(2-NAPHTHALEN-2-YL-1-NAPHTHALEN-1-YL-2-OXO-ETHYL)-PHOSPHONIC 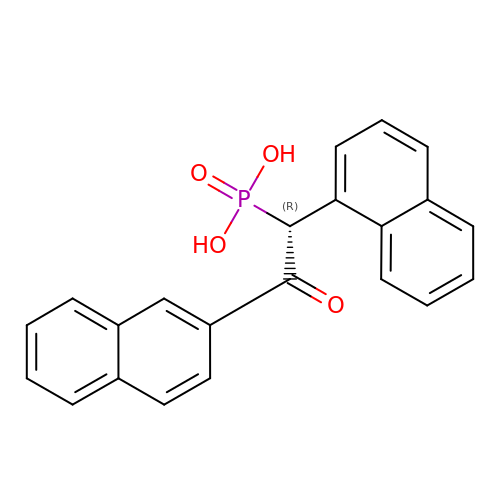ACID | C22 H17 O4 P | OFHMUASCSJJNNA-JOCHJYFZSA-N>MPGSIPLIGERFPEMEVTTDHGVIKLPDHYVSQGKWFVLFSHPADFTPVCTTEFVSFARRYEDFQRLGVDLIGLSVDSVFSHIKWKEWIERHIGVRIPFPIIADPQGTVARRLGLLHAESATHTVRGVFIVDARGVIRTMLYYPMELGRLVDEILRIVKALKLGDSLKRAVPADWPNNEIIGEGLIVPPPTTEDQARARMESGQYRSLDWWFCWDTPASRDDVEEARRYLRRA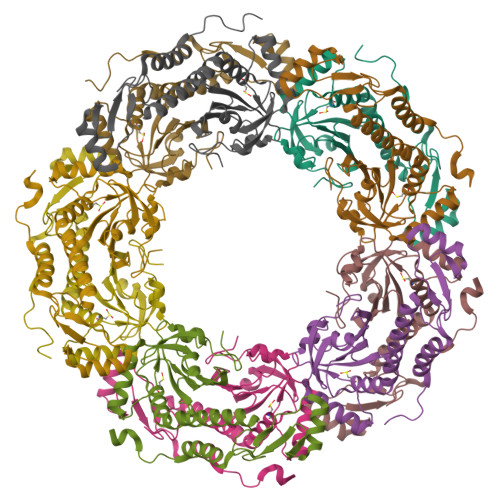AEKPAKLLYEEARTHLH[10x]2-(diethylamino)ethyl 4-((3-(4-nitrophenyl)-3-oxopropyl)amino)benzoate | C22 H27 N3 O5 | 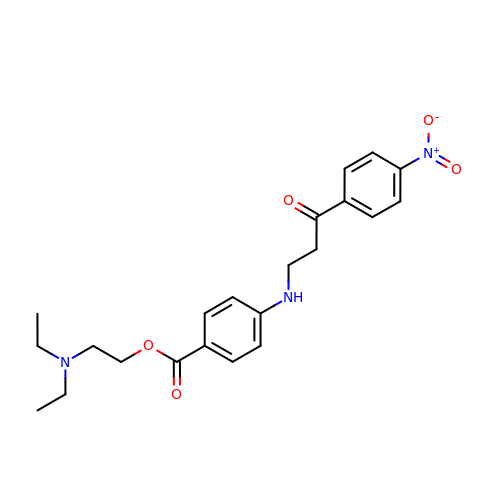GUFSHTOIIPHZRF-UHFFFAOYSA-N O-[(2R,3S,4R,5R)-5-(4-amino-2-oxopyrimidin-1(2H)-yl)-4-hydroxy-2-(hydroxymethyl)tetrahydrofuran-3-yl] O-{[(2R,3S,4R,5R)-5-(2,4-dioxo-3,4-dihydropyrimidin-1(2H)-yl)-3,4-dihydroxytetrahydrofuran-2-yl]methyl} hydrogen (R)-phosphorothioate 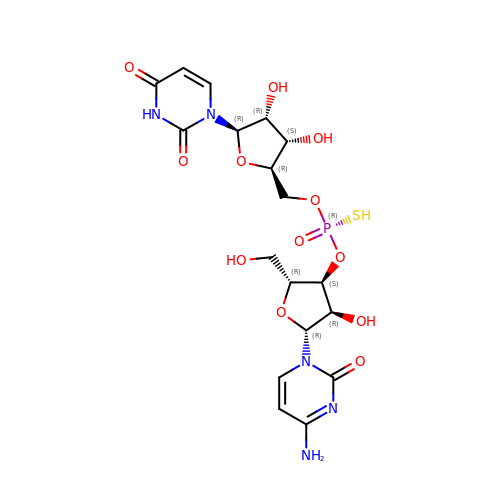| C18 H24 N5 O12 P S | VZQLNJPTHATNOF-ILIYZMILSA-N> MRGSHHHHHHTDPQGDAAQKTDTSHHDQDHPTFNKITPNLAEFAFSLYRQLAHQSNSTNIFFSPVSIATAFAMLSLGTK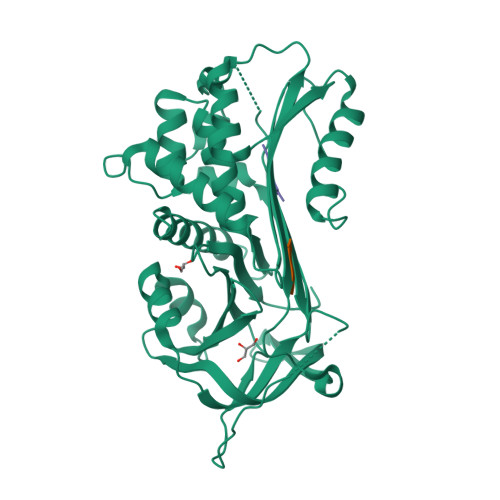ADTHDEILEGLNFNLTEIPEAQIHEGFQELLRTLNQPDSQLQLTTGNGLFLSEGLKLVDKFLEDVKKLYHSEAFTVNFGDTEEAKKQINDYVEKGTQGKIVDLVKELDRDTVFALVNYIFFKGKWERPFEVKDTEEEDFHVDQVTTVKVPMMKRLGMFNIQHCKKLSSWVLLMKYLGNATAIFFLPDEGKLQHLENELTHDIITKFLENEDRRSASLHLPKLSITGTYDLKSVLGQLGITKVFSNGADLSGVTEEAPLKLSKAVHKAVLTIDEKGTEAAGAMFLEAIPMSIPPEVKFNKPFVFLMIEQNTKSPLFMGKVVNPTQK> SVKSEYAEAAAVGQEAVAVFNTMKAAFQNGDKEAVAQYLARLASLYTRHEELLNRILEKARREGNKEAVTLMNEFTATFQTGKSIF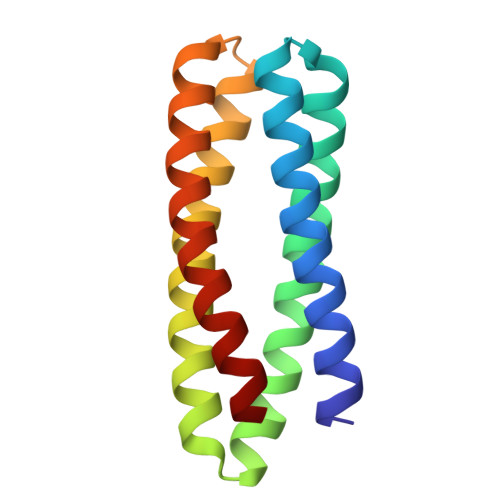NAMVAAFKNGDDDSFESYLQALEKVTAKGETLADQIAKAL>MKHHHHHHHHGGLVPRGSHGGSTIVQELDQAGITDSGLRADYITVSRLFREIGRGRYLGRYMFPAAKRPYFDAFITFVAYVDNLTDDIKHSVEVRARRLDEWERTYLAVAKGDAPSADRPLSRSEQTDAAVARALVHTLRTWDLPYLRVPEFVDGNRKALTTYEYANDEALDEFLETVTLLPAVWINQIFEPRSAEAEELCRHTITAFQLLDFIWDLREDLDLGRLYLPMEHLDRFGVTRADLDRQIGSGHLTDDVRELLRFEIGRAKKHLDAGRGWPQSL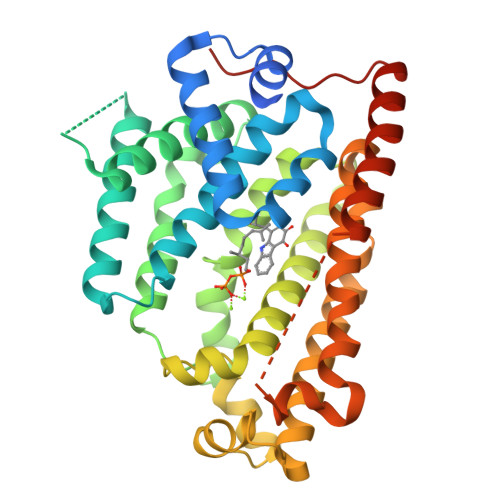HPTSRTFMEADIQLHDSMFPQLTKNGYAFFKTAKAGLGLTSGLMIARTASAIARARKINQQAIRGGYRVRAPFQDGVTE[2x]>NPTSLTDVRVDKAVNFIKPEVSGVAEIQTVTGLSPSTSYLLTPAFLEQNFQSEAGIYILSATPVEGEGTISINMDPTVTTVSGFIKVKTDTFGTFDLSVVLTTASKKQTTGFNIIAATS[2x]

A major factor that limits the expansion of shrimp cultures is, however, infectious diseases from viruses, such as P. vannamei nodavirus (PvNV) and M. rosenbergii nodavirus (MrNV), which have inflicted heavy economic losses. The Nodaviridae genome comprises two single-stranded positive-sense RNA that encode the capsid protein for viral capsid assembly, the RNA polymerase for RNA replication, and the B2 protein for host RNA interference suppressor. While the shell domains (S-domains) of PvNV and MrNV contain conserved sequences of 62% identity, the protrusion domains (P-domains) and N-arms show low sequence identities of only 17% and 43%, respectively. In this work, we have determined the cryo-EM structures of T = 3 and T = 1 PvNV-LPs at atomic resolution, the crystal structures of the P-domains of PvNV and MrNV (PvNVPd and MrNVPd), and the crystal structure of the S-domain of PvNV (ΔN-ARM-PvNVSd) in the T = 1 subviral particle (SVP).

The PvNVPd forms dimers in two crystal forms with the asymmetric unit containing one dimer (space group P21) and two dimers (P212121). The PvNVPd structure (P21) were first determined using Se-Met-derivatized crystals with single-wavelength anomalous diffraction (SAD). All structures of the PvNVPd were refined to resolutions 1.17–1.22 Å. The structures of PvNVPd from two crystal forms are similar with a root mean square deviation (RMSD) < 0.3 Å; and residues 250–368 were resolved in both structures. The structural fold of the PvNVPd consists of eight β-strands, differing from that of any other known viral capsid protein. The P-domain monomer folds into the core jelly-roll topology, forming a β-sandwich face-to-face with two pairs of antiparallel β-sheet. Four highly exposed turn insertions β1/β2, β3/β4, β5/β6, and β7/β8 appear on the top regions of the PvNVPd and might play an important role in the determination of the antigenicity. The semi-flexible N-terminal linker (residues 250–255) located beneath the P-domain must be disordered as there is absence of electron density. In the dimeric structures of PvNVPd and MrNVPd, the domain–domain contacts at the interface are 2-fold symmetrically formed with a hydrogen-bond network between the main chains of the antiparallel β-strands, β3 and β6. Notably, the sequence of the interaction region (Gln273–Asp278) of MrNVPd is distinct from that of PvNVPd, and two types (P21 and P212121) of PVNVPd structures do not exhibit the X-shaped conformation.>MIFTNAILVISALLPATVLSLQHTEDSLFPARCWPDPCAGITFQNDTYVCGDPRLGPVVLPQKFPLNNELRTYARFGALCPAEFLDKWATDVAPNGTYIYPPANGFALDTEEQPILGNATLPVGMKLDRFGSEYGTFLAPLGAPYIERSLPPSNLNTFDGMYPYNYHVYQVTKEFVVGLGPIAPWFEQPGMGTQFVTYTNVLGLIDDGYLRREDPQRLVPRNYGTDVLFQGPGHHHHHH[4x]

The majority of cellular NAD+ is generated in the salvage pathway, where the Nam released in signaling reactions is resynthesized into NAD+.4 Given its importance, NAD+ is targeted by toxins from many pathogenic microorganisms, including Streptococcus pyogenes and Mycobacterium tuberculosis. These toxins invade cells and act as NAD glycohydrolases, cleaving NAD+ into Nam and ADPR and rapidly depleting the cellular NAD pool, ultimately leading to cell death. In this context, we recently discovered a new fungal NADase on the surface of conidia from Aspergillus fumigatus (AfNADase), the predominant etiologic agent of Aspergillosis. The catalytic part of the TNT is structurally highly similar to AfNADase. Intriguingly, the active site architecture of the bacterial and fungal enzymes is conserved, but their structural superimposition reveals the presence of a unique C-terminal calcium-binding motif in AfNADase, which is located at the edge of the dimerization interface. In the present study, we addressed the structural and functional role of calcium binding by introducing mutations in the C-terminus of AfNADase that precluded the binding of the metal ion.

In the second variant, we created a chimeric NADase by replacing the 10 C-terminal amino acids, including the Ca2+-binding motif, with the C-terminus from N. crassa NADase (NcNADase). Importantly, NcNADase lacks the calcium binding site and as a result the chimeric protein, here referred to as AfNADase NcC-Term, is predicted to be unable to bind calcium. Compared to the wild-type enzyme, AfNADase NcC-Term showed a 5-fold decrease in affinity and a 66-fold reduced conversion rate (KM of 272.8 ± 48.6 μM and a Vmax of 69.8 ± 5.3 μmol/min/mg). In contrast, AfNADase NcC-Term showed a large shift in TM, from 71.4 to 57.9 °C for the wild-type and NcC-Term, respectively. These data suggest that at least in the AfNADase NcC-Term, the overall stability of the protein is affected by the modification of the C-terminus that eliminates the calcium binding site. The structure was chosen for the analysis based on the hypothesis that it represents a static conformation resembling dimer 2 of AfNADaseD219A/E220A. In line with this suggestion, the AfNADase NcC-Term variant (dimer 2-like), which lacks the ability to form the native-like C-terminal conformation, exhibits substantially decreased catalytic activity and thermostability.>MPKIVVVGAVAGGATCASQIRRLDKESDIIIFEKDRDMSFANCALPYVIGEVVEDRRYALAYTPEKFYDRKQITVKTYHEVIAINDERQTVSVLNRKTNEQFEESYDKLILSPGASANSLGFESDITFTLRNLEDTDAIDQFIKANQVDKVLVVGAGYVSLEVLENLYERGLHPTLIHRSDKINKLMDADMNQPILDELDKREIPYRLNEEINAINGNEITFKSGKVEHYDMIIEGVGTHPNSKFIESSNIKLDRKGFIPVNDKFETNVPNIYAIGDIATSHYRHVDLPASVPLAWGAHRAASIVAEQIAGNDTIEFKGF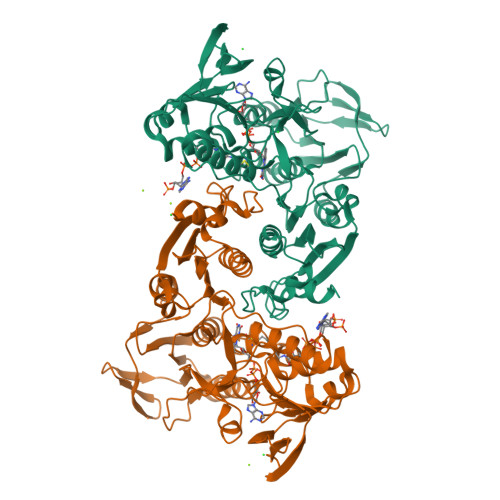LGNNIVKFFDYTFASVGVKPNELKQFDYKMVEVTQGAHANYYPGNSPLHLRVYYDTSNRQILRAAAVGKEGADKRIDVLSMAMMNQLTVDELTEFEVAYAPPYSHPKDLINMIGYKAK[2x]> SVHVPGPHAMTIQELVDYVNARQKQGIYEEYEDIRRENPVGTFHCSMSPGNLEKNRYGDVPCLDQTRVKLTKRSGHTQTDYINASFMDGYKQKNAYIGTQGPLENTYRDFWLMVWEQKVLVIVMT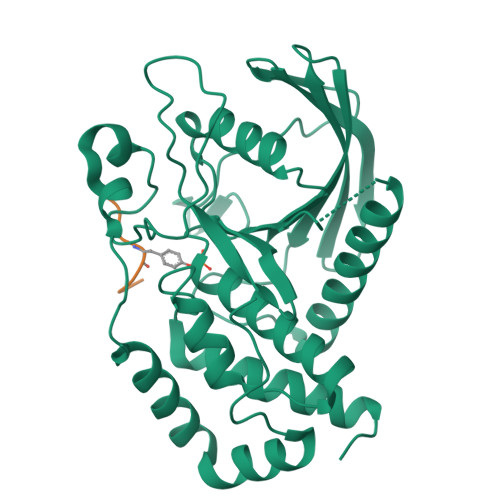TRFEEGGRRKCGQYWPLEKDSRIRFGFLTVTNLGVENMNHYKKTTLEIHNTEERQKRQVTHFQFLSWPAYGVPSSAASLIDFLRVVRNQQSLAVSNMGARSKGQCPEPPIVVHASAGIGRTGTFCSLDICLAQLEELGTLNVFQTVSRMRTQRAFSIQTPEQYYFCYKAILEFAEKEGMVSS;> ESQVYSLDS>[2x]GPLGSVRDEIRSMVSDSVDEIVDGVSKTTAEVINGRKSIAQYATSLIESNPEPDNVRTIISQPLIKNTFLLVGFGLEKDGSNINNDPSWNPGPTWDPRVRPWYKDAKNAGKLVITAPYADSASGEILVSVATPVKDSATGQFLGSIFYDVSLAELAELVNEVKLFDAGYVFIVSEDGTTIAHPKKEFNGKPMSEFLGESKINVDTHQVIINGKPYAVSFSDVEGEDWYVGVVIDEEIAYAALDELRRSTLIHHHHHH

Extracellular signals are sensed by methyl-accepting chemotaxis proteins (MCPs), also known as chemoreceptors. Indeed, we found that Mlp37, the closest homolog of Mlp24, serves as a chemoreceptor for taurine as well as serine, arginine and other amino acids. We determined the crystal structures of the ligand-binding domain of Mlp37 in complex with l-serine and taurine to reveal the molecular mechanism enabling Mlp37 to accommodate these structurally distinct ligands, l-serine and taurine. The ligand complex structures and the mutational analyses demonstrate that only one of the two potential ligand-binding pockets (the membrane-distal pocket I) is involved in ligand binding by Mlp37.

The titration curves of purified Mlp37p (10 μM) with taurine show direct binding with a dissociation constant (Kd) of 3.2 μM, calculated by assuming that an Mlp37p monomer binds one taurine molecule. The taurine complex, like the l-alanine complex, forms a dimer with a neighbouring molecule in the asymmetric unit. Taurine and l-serine are bound only in pocket I in the crystal structures. The binding of taurine is remarkably similar to that of l-serine. The amino group of taurine lies at the equivalent position of that of l-serine and interacts with Tyr-170, Asp-201 and Asp-172. Two oxygen atoms of the sulfonate group are located in the corresponding positions to the carboxyl oxygen atoms of l-serine, but they are out from the plane formed by the guanidino group of Arg-152. Thus, the indole NH of Trp-147 seems to contribute to the interaction in conjunction with the guanidino group of Arg-152, the indole NH of Trp-154 and the main-chain amino group of Ser-173. The remaining oxygen of the sulfonate is located near the hydroxyl oxygen of l-serine, and it interacts with the indole NH of Trp-147 and a water molecule bound to Asp-172, the indole NH of Trp-141, and the main-chain amino group of Ala-174. These structural features are essentially the same in the two subunits of the dimeric Mlp37p taurine complex. The residues in contact with taurine can be superimposed onto the corresponding residues of the l-serine complex, with root mean square deviations of about 0.3 Å (0.314 for A-subunit and 0.265 for B-subunit), indicating that taurine mimics l-serine in Mlp37.> MGRAFEYRRAAKEKRWDKMSKVFPKLAKAITLAAKDGGSEPDTNAKLRTAILNAKAQNMPKDNIDAAIKRASSKEGNLSEITYEGKANFGVLIIMECMTDNPTRTIANLKSYFNKTQGASIVPNGSLEFMFNRKSVFECLKNEVENLKLSLEDLEFALIDYGLEELEEVEDKIIIRGDYNSFKLLNEGFESLKLPILKASLQRIATTPIELNDEQME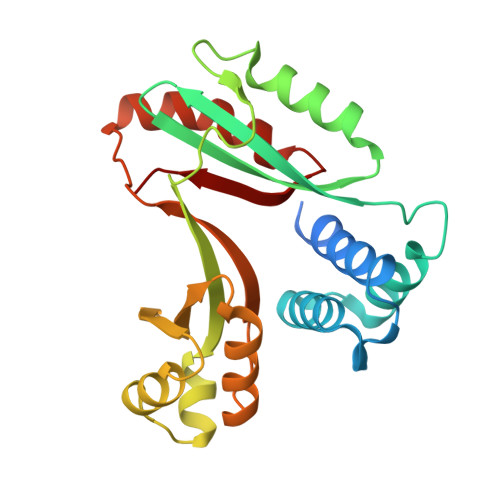LTEKLLDRIEDDDDVVALYTNIE> XT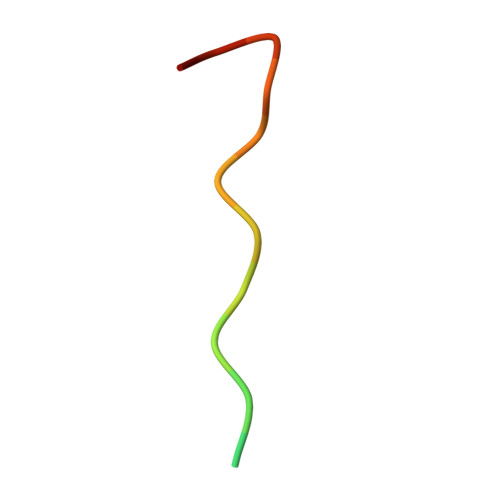RRRRKLPEIPKNKKX>MGSSHHHHHHSSGRENLYFQGMELLKHLSQRQYIDGEWVESANKNTRDIINPYNQEVIFTVSEGTKEDAERAILAARRAFESGEWSQETAETRGKKVRAIADKIKEHREALARLETLDTGKTLEESYADMDDIHNVFMYFAGLADKDGGEMIDSPIPDTESKIVKEPVGVVTQITPWNYPLLQASWKIAPALATGCSLVMKPSEITPLTTIRVFELMEEVGFPKGTINLILGAGSEVGDVMSGHKEVDLVSFTGSIETGKHIMKNAANNVTNIALELGGKNPNIIFDDADFELAVDQALNGGYFHAGQVCSAGSRILVQNSIKDKFEQALIDRVKKIKLGNGFDADTEMGPVISTEHRNKIESYMDVAKAEGATIAVGGKRPDRDDLKDGLFFEPTVITNCDTSMRIVQEEVFGPVVTVEGFETEQEAIQLANDSIYGLAGAVFSKDIGKAQRVANKLKLGTVWINDFHPYFAQAPWGGYKQSGIGRELGKEGLEEYLVSKHILTNTNPQLVNWFSK[8x]

We studied a putative BADH from an early MRSA COL isolate, denoted SaBADH, and showed that it is a functional NAD+-dependent BADH that utilizes BA as the primary substrate. BADHs are a group of enzymes from the aldehyde dehydrogenase (ALDH) superfamily that primarily catalyze the oxidation of betaine aldehyde (BA) to betaine; some BADHs also utilize other substrates. BADHs resemble ALDH in structure and are composed of a Rossmann-fold NAD(P)-binding domain, a catalytic (substrate-binding) domain and an oligomerization (bridging) domain. The solution data are supported by the structural analysis and emphasize the importance of the NAD+-driven structural rearrangements at the cofactor-binding and substrate-binding sites for enzymatic activity.

We previously showed that the substitution of Gly234, which is located in the NAD-binding area, by a serine residue increased the affinity of SaBADH for NAD+ and made the mutant more active than the wild type. The mutation also reduced the substrate inhibition. To fully understand the kinetic and inhibition mechanisms of G234S-SaBADH, we determined its crystal structures in apo and holo forms and in the presence/absence of BME and compared them with the wild-type structures. The BME–Cys289 adduct and the G234S mutation determine the NAD-binding mode in SaBADH. In NAD–G234S-SaBADHBME(−), the dinucleotide is in the ‘hydride-transfer’ position, in which the amide group of NMN displaces the γ-carboxyl group of the catalytic base Glu255 towards its single ‘intermediate’ conformation. The lack of a serine residue at position 234, which stabilizes the ‘hydride-transfer’ position of NAD+ in NAD–G234S-SaBADHBME(−), may also account for the observed flexibility of NAD+ in NAD–SaBADHBME(−). When the NAD–G234S-SaBADHBME(−) and NAD–SaBADHBME(−) structures were superimposed, the NAD+ ‘hydride-transfer’ conformer of the former structure fitted the aforementioned uncertain electron density of the latter structure. Thus, BME oxidation of Cys289 and the G234S mutation helped to trap the ‘hydrolysis’ and ‘hydride-transfer’ positions of the cofactor, respectively, allowing analysis of these binding modes in SaBADH.> QFIA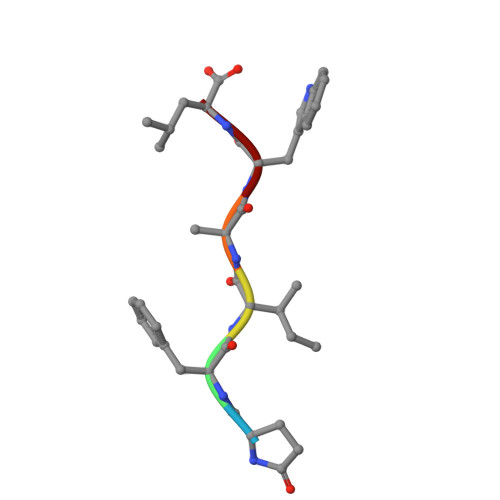WL>[2x]MRSRR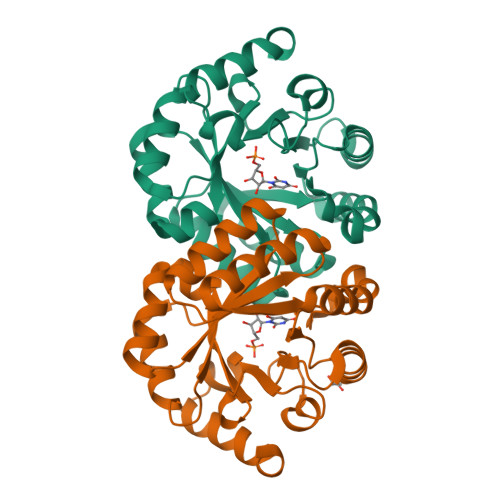VDVMDVMNRLILAMDLMNRDDALRVTGEVREYIDTVKIGYPLVLSEGMDIIAEFRKRFGCRIIADFKVADIPETNEAICRATFKAGADAIIVHGFPGADSVRACLNVAEEMGREVFLLTEMSHPGAEMFIQGAADEIARMGVDLGVKNYVGPSTRPERLSRLREIIGQDSFLISPGVGAQGGDPGETLRFADAIIVGRSIYLADNPAAAAAGIIESIKDLLNP> NLVQFGVMIEKMTGKSALQYNDYGCYCGIGGSHWPVDQTDWCCHAH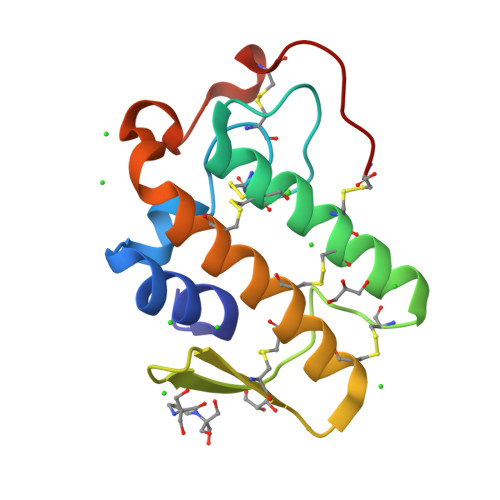DCCYGRLEKLGCEPKLEKYLFSVSERGIFCAGRTTCQRLTCECDKRAALCFRRNLGTYNRKYAHYPNKLCTGPTPPC5-O-phosphono-D-ribonic acid | C5 H11 O9 P | 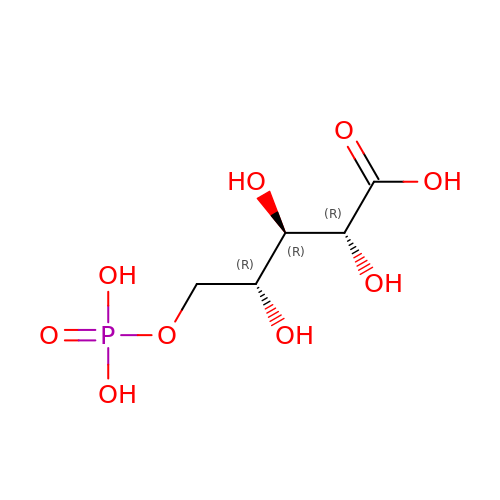HNECGPFIYSOYHF-BXXZVTAOSA-N3-{[4-(trifluoromethyl)phenyl]amino}benzoic 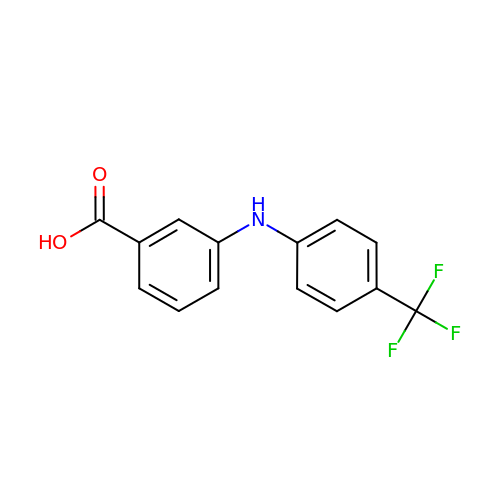acid | C14 H10 F3 N O2 | MDZIRNPRVJEHHX-UHFFFAOYSA-N> PQYGIAREDVVLNRILGEGFFGEVYEGVYTNHKGEKINVAVKTCKKDCTLDNKEKFMSEAVIMKNLDHPHIVKLIGIIEEEPTWIIMELYPYGELGHYLERNKNSLKVLTLVLYSLQICKAMAY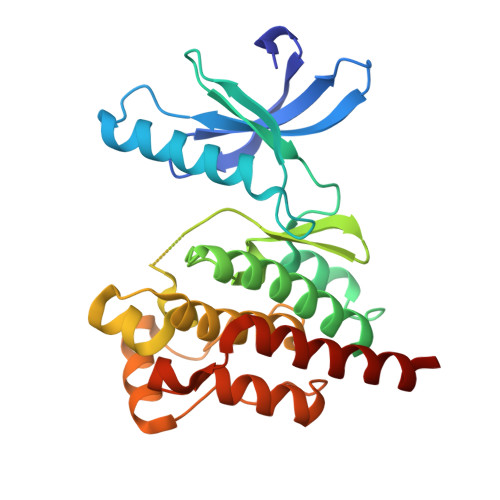LESINCVHRDIAVRNILVASPECVKLGDFGLSRYIEDEDYYKASVTRLPIKWMSPESINFRRFTTASDVWMFAVCMWEILSFGKQPFFWLENKDVIGVLEKGDRLPKPDLCPPVLYTLMTRCWDYDPSDRPRFTELVCSLSDVYQMEKDIAME>MHH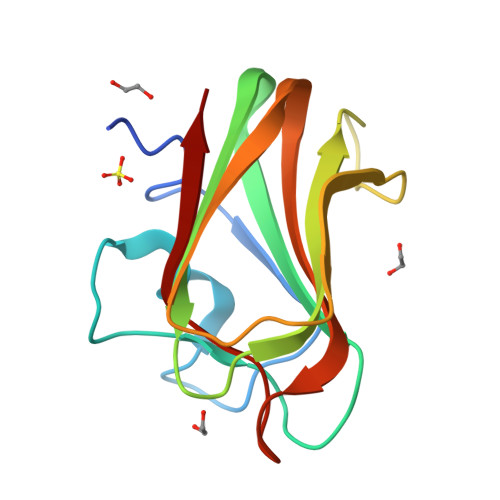HHHHNLALNKTATASSIEGAGFEASRAFDGSSTTRWASAEGVDPQWIYVNLGSSQTVNRVKLNWEAAYASSYTIQVSNDSGTPTNWTTVYTTTTGDGGIDDITFTARTAKYVRVHGTVRGTPYGYSLWEFEVYG[3x]The Drosophila tumour necrosis factor (TNF) ligand-receptor system consists of a unique ligand, Eiger (Egr), and two receptors, Grindelwald (Grnd) and Wengen (Wgn), and therefore provides a simple system for exploring the interplay between ligand and receptors, and the requirement for Grnd and Wgn in TNF/Egr-mediated processes. Here, we report the crystallographic structure of the extracellular domain (ECD) of Grnd in complex with Egr, a high-affinity hetero-hexameric assembly reminiscent of human TNF:TNFR complexes. Here we show that trimeric Egr ligands assemble in hetero-hexamers with both Grnd and Wgn, with Grnd displaying nanomolar binding affinity for Egr, which is 3-orders of magnitude higher than that for Wgn. Altogether, our data provide insight into ligand-mediated activation of Grnd and suggest that distinct affinities of TNF ligands for their receptors promote different and non-redundant cellular functions.

To shed light on the mechanism of Grnd activation by Egr, we set out to determine the crystallographic structure of the complex. To obtain diffraction-quality crystals, the Grnd30–97:Egr146–409 sample was subjected to limited proteolysis, yielding shorter constructs assigned by mass spectrometry to Egr269–409 and Grnd30–81, that still form complexes in solution according to SEC analysis. Grnd30–81:Egr269–409 crystals diffracted to a resolution of 2.02 Å and belonged to the P321 space group, reflecting the threefold symmetry axis observed in the complex. The final model includes residues 269–409 of Egr and amino acids 31–81 of Grnd. The architecture of the hetero-hexameric complex consists of a core Egr trimer bound to three Grnd-ECD copies positioned distally. No major conformational rearrangements of the Grnd fold can be observed upon binding to its ligand Egr (with a rmsd of 0.674 Å between the free and bound state), that associates as rigid bodies with no induced fit. Importantly, in the Egr:Grnd arrangement each copy of Grnd contacts two Egr protomers, implying that the trimeric state of the ligand is essential for the organisation of the high-affinity interaction surface with the receptor. The TNF domain of Egr adopts a typical “jelly-roll” fold, with an inner and an outer β-sheet composed of five antiparallel β-strands (conventionally named A’AHCF and B’BGDE, respectively). The interface between Egr and Grnd is organized in three surface patches. The modular interaction surface is provided mainly by the Grnd β-hairpin that snugly fits in between two TNF domains and the α1-α2 loop, strengthening the binding by His66-Asn67Grnd-mediated polar interactions.

> SEDSRPAAHFHLSSRRRHQGSMGYHGDMYIGNDNERNSYQGHFQTRDGVLTVTNTGLYYVYAQICYNNSHDQNGFIVFQGDTPFLQCLNTVPTNMPHKVHTCHTSGLIHLERNERIHLKDIHNDRNAVLREGNNRSYFGIFKV;> GESRDCHGTICHPVNEFCYVATERCHPCIEVCNNQTHNYDAFLCAKECSAYK>MST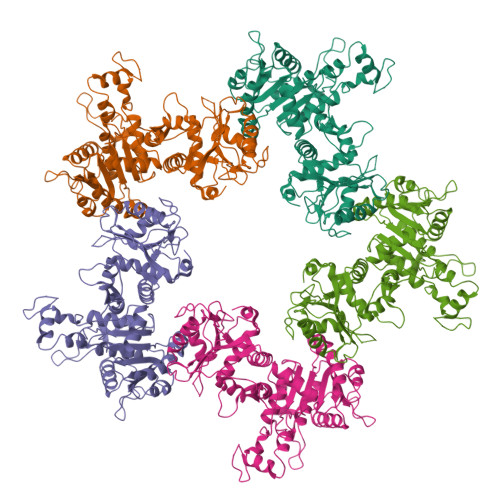QSNRNALVVAQLKGDFVAFLFVLWKALNLPVPTKCQIDMAKVLANGDNKKFILQAFRGIGKSFITCAFVVWSLWRDPQLKILIVSASKERADANSIFIKNIIDLLPFLSELKPRPGQRDSVISFDVGPANPDHSPSVKSVGITGQLTGSRADIIIADDVEIPSNSATMGAREKLWTLVQEFAALLKPLPSSRVIYLGTPQTEMTLYKELEDNRGYTTIIWPALYPRTREENLYYSQRLAPMLRAEYDENPEALAGTPTDPVRFDRDDLRERELEYGKAGFTLQFMLNPNLSDAEKYPLRLRDAIVAALDLEKAPMHYQWLPNRQNIIEDLPNVGLKGDDLHTYHDCSNNSGQYQQKILVIDPSGRGKDETGYAVLYTLNGYIYLMEAGGFRDGYSDKTLELLAKKAKQWGVQTVVYESNFGDGMFGKVFSPILLKHHNCAMEEIRARGMKEMRICDTLEPVMQTHRLVIRDEV[5x]>[4x]MTETYPVVKGAEPFFFEGNDIGILVLHGFTGSPQSMRPLGEAYHEAGYTVCGPRLKGHGTHYEDMEKTTCQDWIDSVEAGYEWLKNRCGTIFVTGLSMGGTLTLYMAEHHPEICGIAPINAAINMPALAGALAGVGDLPRFLDAIGSD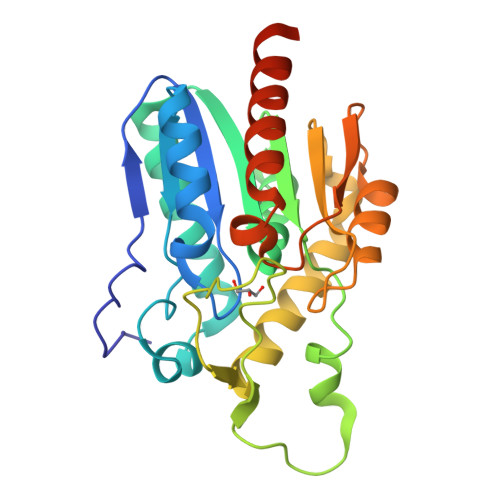IKKPGVKELAYEKTPVKSIGEITELMKKVKGDLEKVNCPALIFVSKEDHVVPPSNSQEIYSSIKSAAKELVTLDNSYHVATLDNDQDIIIERTLHFLQRVLETSSLQGLEHHHHHH> NTTGG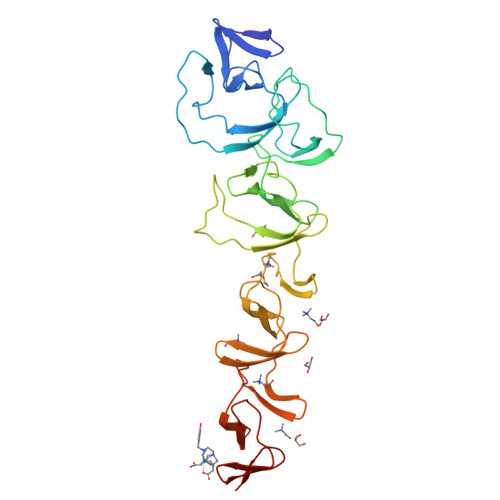RFVDKDNRKYYVKDDHKAIYWHKIDGKTYYFGDIGEMVVGWQYLEIPGTGYRDNLFDNQPVNEIGLQEKWYYFGQDGALLEQTDKQVLEAKTSENTGKVYGEQYPLSAEKRTYYFDNNYAVKTGWIYEDGNWYYLNKLGNFGDDSYNPLPIGEVAKGWTQDFHVTIDIDRSKPAPWYYLDASGKMLTDWQKVNGKWYYFGSSGSMATGWKYVRGKWYYLDNKNGDMKTGWQYLGNKWYYLRSSGAMVTGWYQDGLTWYYLNAGNGDMKTGWFQVNGKWYYAYSSGALAVNTTVDGYSVNYNGEWVQ>[4x]MTSPSSPPAFRLETSDGGQDGAEVDKAQLGYGAGPPPMESRFQDEDRNFPPQIKVNLNYRKGAGASQPDLNRFDRDRLFNVVARGNPEDLAGLLEYLRRTSKYLTDSEYTEGSTGKTCLMKAVLNLQDGVNACIQPLLEIDRDSGNPQPLVNAQCTDEYYRGHSALHIAIEKRSLQCVKLLVENGANVHAKACGHFFQKNQDTCFYFGELPLSLAACTKQWDVVNYLLENPHQPASLQAQDSLGNTVLHALVMIADDSAENSALVVRMYDGLLQAGARLCPNVQLEGIPNLEGLTPLKLAAKEGKIEIFKHILQREFSAPCQSLSRKFTEWCYGPVRVSLYDLASVDSWEENSVLEIIAFHSRSPHRHRMVVLEPLNKLLQAKWDRLIPRFCFNFLCYLVYMLIFTAVAYHQPALEKQGFPPLKATAGNSMLLLGHILILLGGVYLLLGQLWYFWRRRLFIWISFMDSYSEILFLLQALLTVLSQVLCFLAIEWYLPLLVSSLAMGWTNLLYYTRGFQHTGIYSVMIEKVILRDLLRFLLVYLVFLFGFAVALVSLSREAQNSRTPAGPNATEVGQPGAGQEDEAPPYRSILDASLELFKFTIGMGELAFQEQLRFRGVVLLLLLAYVLLTYVLLLNMLIALMSETVNSVATDSWSIWKLQKAISVLEMENGYWWCRRKKQRAGVMLTVGTRPDGSPDERWCFRVGEMNWATWEQTLPRTLCEEPSGAAAPGVMKNPTPASQRGEDSASEEDHLPLQLLQSRSNLEVLFQGPHHHHHHDYKDDDDK

TRPV1-TRPV4 are non-selective cation channels which play important physiological roles in sensing noxious heat, maintaining cardiac structure and maintaining skin, hair and bone physiology. A distinctive feature of TRPV1 and TRPV2 is their permeability to large organic cations, such as the cationic dye YO-PRO-1 and the sodium channel blocker QX-314. The non-conducting structures of TRPV1 and TRPV2 possess two restrictions, one at the selectivity filter (SF) and second one at the intracellular mouth of the pore (termed the common gate). Our data shows that binding of RTx induces C2 symmetric conformations in TRPV2, but the extent of C2 symmetry depends on the environment in which the channel is reconstituted.

Classification of the TRPV2RTx-APOL sample revealed the presence of four classes: one low-resolution (~7 Å) class, which was excluded from further analysis, and three higher resolution classes which are representative of three different conformations. These include one C4 symmetric and two distinct C2 symmetric classes refined to 2.9 Å, 3.3 Å and 4.2 Å, respectively. Unexpectedly, the transmembrane domains (TM) of the three structures obtained from amphipol-reconstituted TRPV2, TRPV2RTx-APOL 1-3, show similarity to our previously solved cryo-EM structure of TRPV2 in its apo form (TRPV2APO) and adopt non-conducting conformations. While fully bound to RTx, the TM domains of TRPV2RTx-APOL 1 and TRPV2RTx-APOL 2 structures largely retain C4 symmetry. In order to determine the effect of RTx on the TRPV2RTx-APOL sample, we aligned TRPV2RTx-APOL 1 with TRPV2APO. The transmembrane helices S1-S6 of the two channels aligned remarkably well (Cα R.M.S.D = 0.86). However, RTx binding induces a 5° clockwise rotation of the ARD when viewed from the extracellular space and a ~ 10 Å lateral widening of the cytoplasmic assembly. In addition, RTx causes a conformational change in the S4-S5 linker, as well as a displacement of the TRP domain. The conformational change in the S4-S5 linker is caused by the introduction of a π-helical turn at the junction of the S4-S5 linker and the S5 helix in the TRPV2RTx-APOL 1 structure (S4-S5π-hinge), which is absent in TRPV2APO (Figure 3—figure supplements 1 and 4). Nevertheless, the RTx-induced conformational changes in the S4-S5 linker are not efficiently propagated to the TM in the TRPV2RTx-APOL structures, and they fail to open either of the two restrictions in the pore.> FSEECMHGSGENYDGKISKTMSGL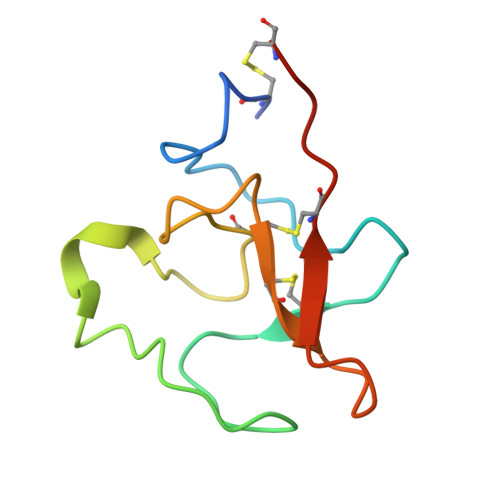ECQAWDSQSPHAHGYIPSKFPNKNLKKNYCRNPDRDLRPWCFTTDPNKRWEYCDIPRCAA>GGVVNPNEVFCSVPGRLSLLSSTSKYKVTVAEVQRRLSPPECLNASLLGGVLRRAKSKNGGRSLREKLDKIGLNLP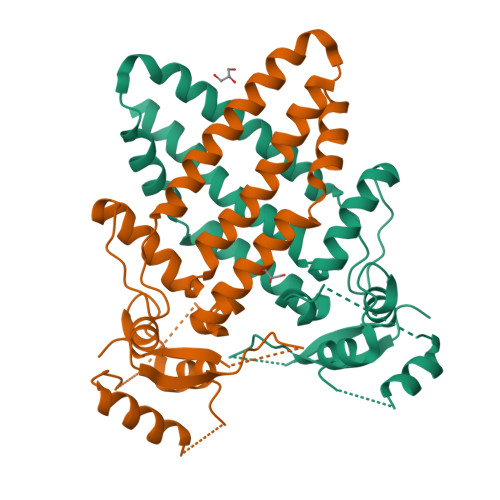AGRRKAANVTLLTSLVEGEAVHLARDFGYVCETEFPAKAVAEFLNRQHSDPNEQVTRKNMLLATKQICKEFTDLLAQDRSPLGNSRPNPILEPGIQSCLTHFNLISHGFGSPAVCAAVTALQNYLTEALKAMDKMYLSNNPNS[2x]> 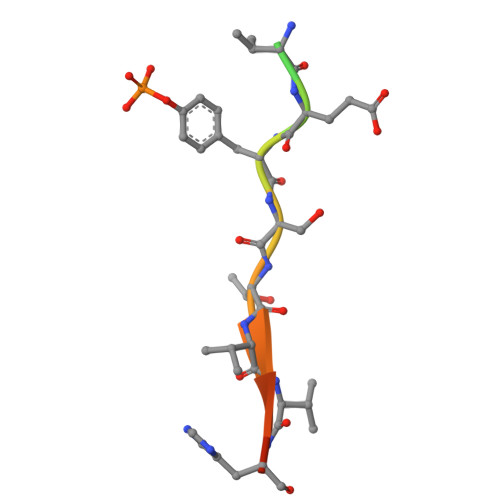STASTVEYSTVVHSG>MFKIGSVLKQIRQELNYHQIDLYSGIMSKSVYIKVEADSRPISVEELSKFSERLGVNFFEILNRAGMNTKSVNETGKEKLLISKIFTNPDLFDKNFQRIEPKRLTSLQYFSIYLGYISIAHHYNIEVPTFNKTITSDLKHLYDKRTTFFGIDYEIVSNLLNVLPYEEVSSIIKPMYPIVDSFGKDYDLTIQTVLKNALTISIMNRNLKEAQYYINQFEHLKTIKNISINGYYDLEINYLKQIYQFLTDKNIDSYLNAVN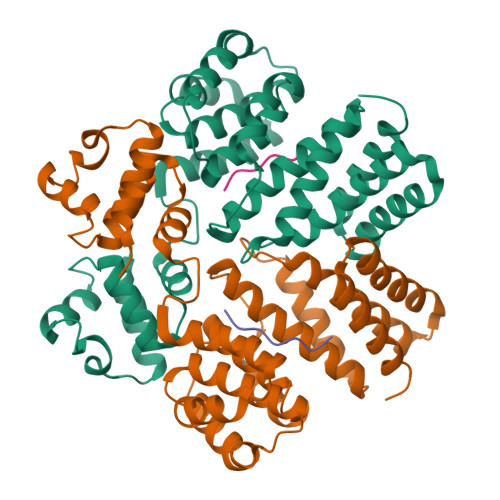IINIFKIIGKEDIHRSLVEELTKISAKEKFTPPKEVTMYYENYVAIENNPIPEIKEQS[2x];>[2x]LVTLVFV>MKVLVTGFEPFGGEKINPTERIAKDLDGIKIGDAQVFGRVLPVVFGKAKEVLEKTLEEIKPDIAIHVGLAPGRSAISIERIAVNAIDARIPDNEGKKIEDEPIVPGAPTAYFSTLPIKKIMKKLHERGIPAYISNSAG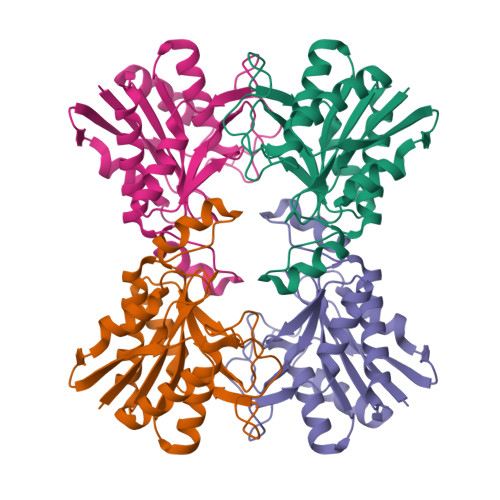LYLSNYVMYLSLHHSATKGYPKMSGFIHVPYIPEQIIDKIGKGQVPPSMSYEMALEAVKVAIEVALEELL[4x]>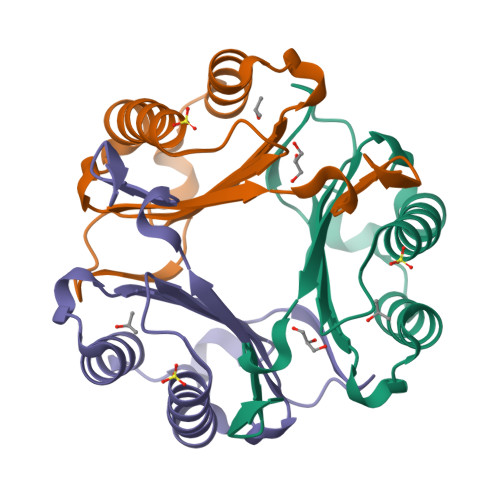[3x]PMFIVNTNVPRASVPDGFLSELTAALAQATGKPPQYIAVHVVPDQLMAFGGSSEPCALCSLHSIGKIGGAQNRSYSKLLCGLLAERLRISPDRVYINYYDMNAANVGWNNSTFA> X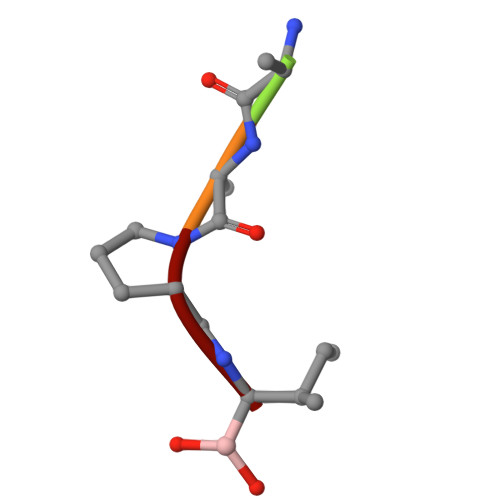AAPI> GSKVEDPKDFPSELLSFLSHAVCSNRTLACFAIYTTKEKAALLYKKIMEKYSVTFISRHNSYNHNILFFLTPHRHRVSAINNYAQKLATFSFLICKGVNKEYLMYSALTRDPFSVIEESLPGGLKEHCFNPESS

The modular multifunctional protein large T antigen (T-ag) from simian virus 40 orchestrates many of the events needed for replication of the viral double-stranded DNA genome. This protein assembles into single and double hexamers on specific DNA sequences located at the origin of replication. T-ag contains three structurally and functionally independent domains: an N-terminal J domain followed by the origin-binding domain (OBD) and the helicase domain. The T-ag OBD has multiple functions; it binds the GAGGC sequences in the origin of replication in a sequence-specific manner.

When the wt T-ag OBD structure was analyzed via the program SSBOND, we identified only one pair as candidates for mutation: Phe151 and Asp256. Therefore, to eliminate disulfide formation with Cys216, we also mutated Cys216 to alanine (Cys216Ala). Finally, using a vector encoding a double mutant of T-ag OBD (pGEX T-ag OBDC216A, F151C), we generated a vector encoding the triple-mutant form T-ag OBDF151C, C216A, D256C (termed 3XM). However, under oxidizing conditions 3XM forms higher order complexes (dimers, trimers etc.) as analyzed by SDS–PAGE. To verify that the desired intermolecular disulfide bond formed between Phe151Cys and Asp256Cys, we crystallized the triple mutant and subjected the crystals to X-ray analysis. The triple mutant crystallized in the same space group (P65) and has almost identical unit-cell parameters as the wt T-ag OBD. The final model contains amino acids 131–252 and 254–257, 127 water molecules and one citrate molecule. Nonetheless, the electron density for the disulfide bond connecting the protomers is clear. Despite the indicated changes, the backbones of the two structures are virtually identical. Finally, although the triple mutant has reorganized a portion of the protein–protein interface, the disulfide cross-link, together with the other protein–protein interactions, are sufficient for formation of the crystallographic hexamer.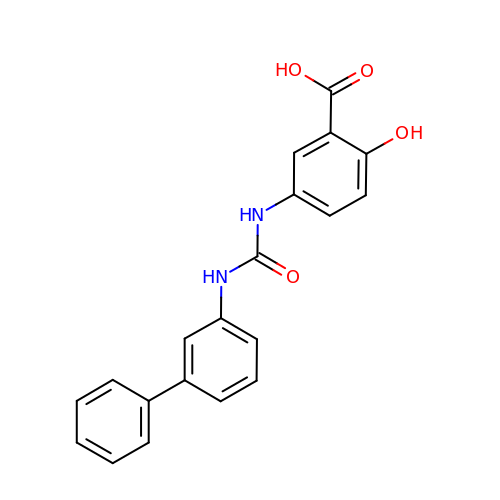5-{[([1,1'-biphenyl]-3-yl)carbamoyl]amino}-2-hydroxybenzoic acid | C20 H16 N2 O4 | BRISALGJKGCDGB-UHFFFAOYSA-N>MSDTMVVNGSGGVPAFLFSGSTLSSYRPNFEANSI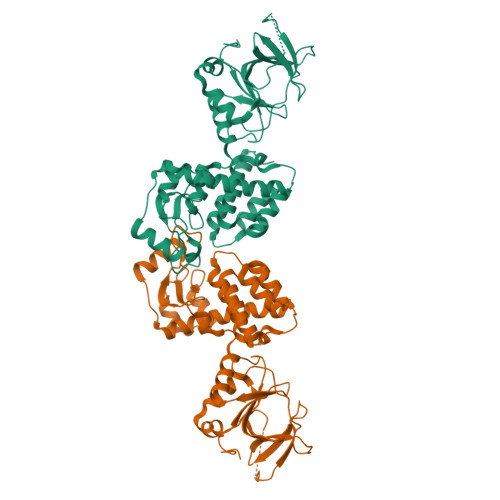TIALPHYVDLPGRSNFKLMYIMGFPIDTEMEKDSEYSNKIRQESKISKTEGTVSYEQKITVETGQEKDGVKVYRVMVLEGTIAESIEHLDKKENEDILNNNRNRIVLADNTVINFDNISQLKEFLRRSVNIVDHDIFSSNGFEGFNPTSHFPSNPSSDYFNSTGVTFGSGVDLGQRSKQDLLNDGVPQYIADRLDGYYMLRGKEAYDKVRTAPLTLSDNEAHLLSNIYIDKFSHKIEGLFNDANIGLRFSDLPLRTRTALVSIGYQKGFKLSRTAPTVWNKVIAKDWNGLVNAFNNIVDGMSDRRKREGALVQKDIDSGLLK[2x]>[6x]VIRHFLRDD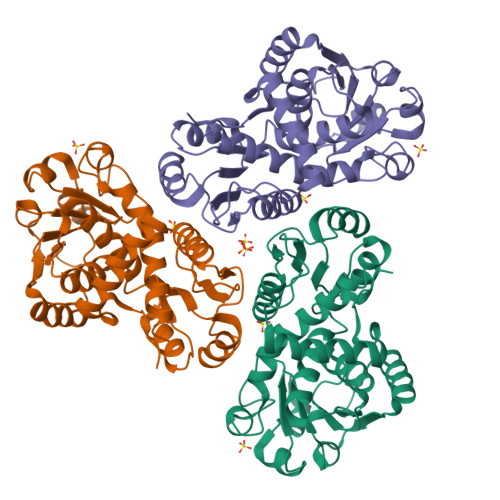DLSPAEQAEVLELAAELKKDPVSRRPLQGPRGVAVIFDKNSTRTRFSFELGIAQLGGHAVVVDSGSTQLGRDETLQDTAKVLSRYVDAIVWRTFGQERLDAMASVATVPVINALSDEFHPCQVLADLQTIAERKGALRGLRLSYFGDGANNMAHSLLLGGVTAGIHVTVAAPEGFLPDPSVRAAAERRAQDTGASVTVTADAHAAAAGADVLVTDTWTSMGQENDGLDRVKPFRPFQLNSRLLALADSDAIVLHCLPAHRGDEITDAVMDGPASAVWDEAENRLHAQKALLVWLLERS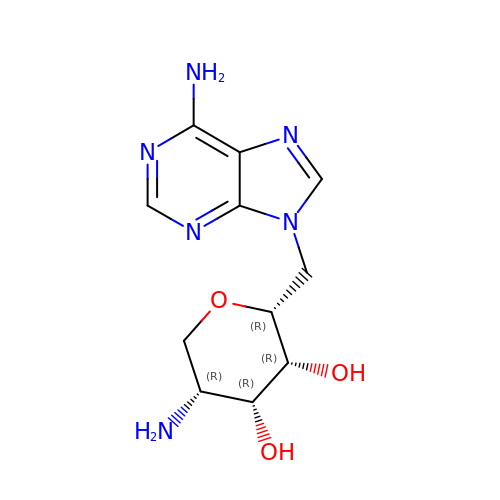(2~{R},3~{R},4~{R},5~{R})-2-[(6-aminopurin-9-yl)methyl]-5-azanyl-oxane-3,4-diol | C11 H16 N6 O3 | YFNWLMALNRKCLH-GCXDCGAKSA-N> GSAMGSTSRKKVLLKVIILGDSGVGKTSLMNQYVNKKFSNQYKATIGADFLTKEVMVDDRLVTMQIWDTAGLERFQSLGVAFYRGADCCVLVFDVTAPNTFKTLDSWRDEFLIQASPRDPENFPFVVLGNKIDLENRQVATKRAQAWCYSKNNIPYFETSAKEAINVEQAFQTIARNALKQET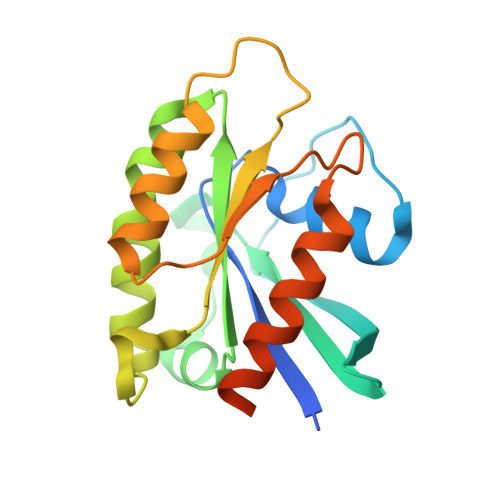EVELYNEFPEPIKLDKN> PATPTASS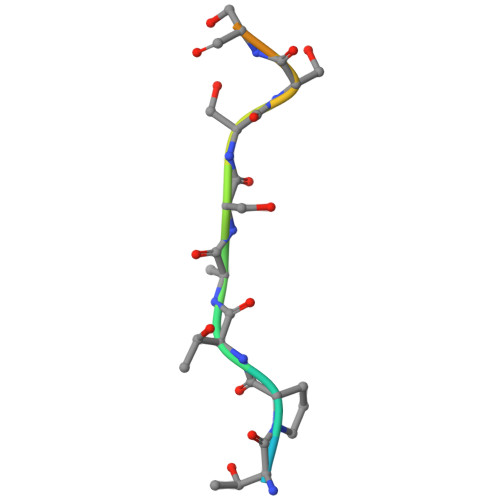SSSTTPT>MAMSQQDLPTLFYSGKSNSAVPIISESELQTITAEPWLEISKKGLQLEGLNFDRQGQLFLLDVFEGNIFKINPETKEIKRPFVSHKANPAAIKIHKDGRLFVCYLGDFKSTGGIFAATENGDNLQDIIEDLSTAYCIDDMVFDSKGGFYFTDFRGYSTNPLGGVYYVSPDFRTVTPIIQNISVANGIALSTDEKVLWVTETTANRLHRIALEDDGVTIQPFGATIPYYFTGHEGPDSCCIDSDDNLYVAMYGQGRVLVFNKRGYPIGQILIPGRDEGHMLRSTHPQFIPGTNQLIICSNDIEM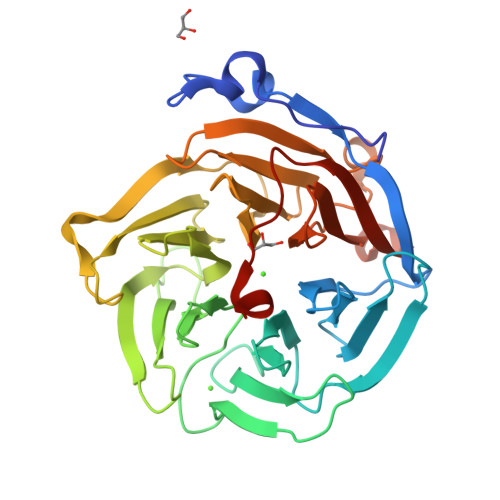GGGSMLYTVNGFAKGHQSFQFQLEHHHHHH[6x]>[4x]AMMKAAVVRAFGAPLTIDEVPVPQPGPGQVQVKIEASGVCHTDLHAADGDWPVKPTLPFIPGHE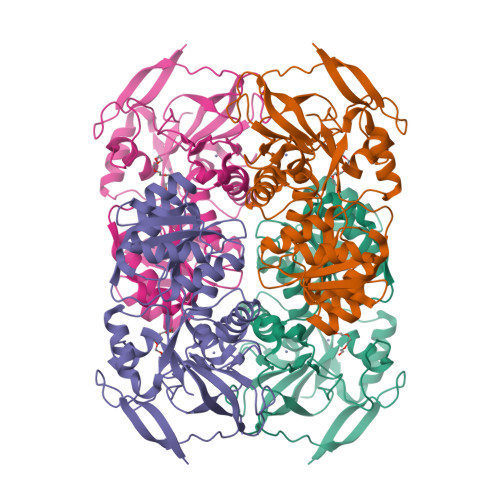GVGYVSAVGSGVSRVKEGDRVGVPWLYSACGYCEHCLQGWETLCEKQQNTGYSVNGGYGEYVVADPNYVGLLPDKVGFVEIAPILCAGVTVYKGLKVTDTRPGQWVVISGIGGLGHVAVQYARAMGLRVAAVDIDDAKLNLARRLGAEVAVNARDTDPAAWLQKEIGGAHGVLVTAVSPKAFSQAIGMVRRGGTIALNGLPPGDFGTPIFDVVLKGITIRGSIVGTRSDLQESLDFAAHGDVKATVSTAKLDDVNDVFGRLREGKVEGRVVLDFSR>EAEAEFSVSYDDRAIIINGKRKILISGSIHYPRSTPQMWPDLIQKAKDGGLDVIETYVFWNGHEPSPGKYNFEGRYDLVRFIKMVQRAGLYVNLRIGPYVCAEWNFGGFPVWLKYVPGMEFRTNNQPFKVAMQGFVQKIVNMMKSENLFESQGGPIIMAQIENAYGPVEWEIGAPGKAYTKWAAQMAVGLKTGVPWIMCKQEDAPDPVIDTCNGFYCEGFRPNKPYKPKMWTEVWTGWYTKFGGPIPQRPAEDIAFSVARFVQNNGSFFNYYMYHGGTNFGRTSSGLFIATSYDYDAPLDEYGLLNEPKYGHLRDLHKAIKLSEPALVSSYAAVTSLGSNQEAHVYRSKSGACAAFLSNYDSRYSVKVTFQNRPYNLPPWSISILPDCKTAVYNTAQVNSQSSSIKMTPAGGGLSWQSYNEETPTADDSDTLTANGLWEQKNVTRDSSDYLWYMTNVNIASNEGFLKNGKDPYLTVMSAGHVLHVFVNGKLSGTVYGTLDNPKLTYSGNVKLRAGINKISLLSVSVGLPNVGVHYDTWNAGVLGPVTLSGLNEGSRNLAKQKWSYKVGLKGESLSLHSLSGSSSVEWVRGSLMAQKQPLTWYKATFNAPGGNDPLALDMASMGKGQIWINGEGVGRHWPGYIAQGDCSKCSYAGTFNEKKCQTNCGQPSQRWYHVPR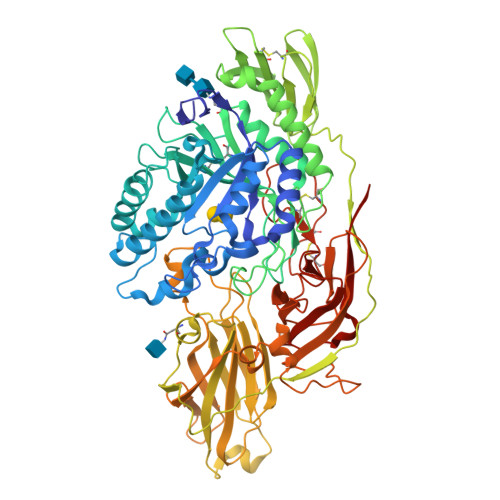SWLKPSGNLLVVFEEWGGNPTGISLVRRSRSAAAASFLEQK[2x]> SLRYSRHDGTSCVIDNHHLKSLGAVLNDVRRKKDRIREAEYEPIIDIADQYMVTEDPFRGPGKNVRITLFKEIRRVHPDTMKLVCNWSGKEFLRETWTRFISEEFPITTDQEIMDLWFELQLRPMHPNRCYKFTMQYALGAHPDYVAHDVIRQ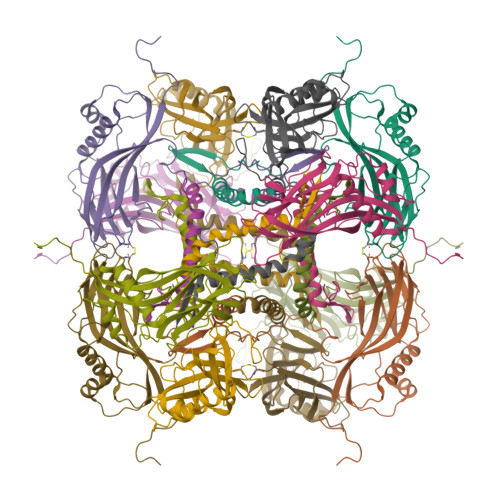QDPYYVGPNNIERINLSKKGFAFPLTCLQSVYNDNFERFFDDVLWPYFYRPLVYVGTTSAEIEEIMIEVSLLFKIKEFAPDVPLFTGPAY>N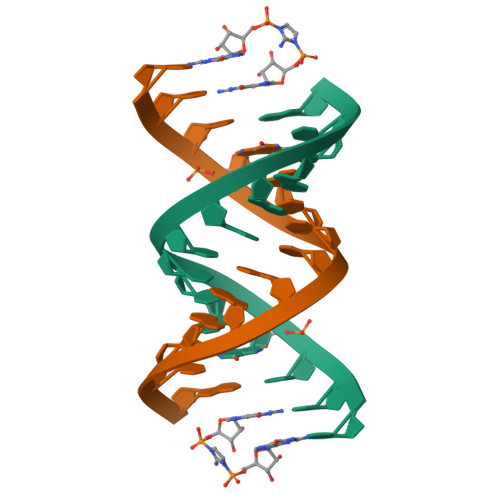NNGACUUAAGUCG[2x]>[4x]HHHHHHMSAIKPDMKINLRMEGNVNGHHFVIDGDGTGKPFEGKQSMDLEVKEGGPLPFAFDILTTAFHYGNRVFAEYPDHIQDYFKQSFPKGYSWERSLTFEDGGICIARNDI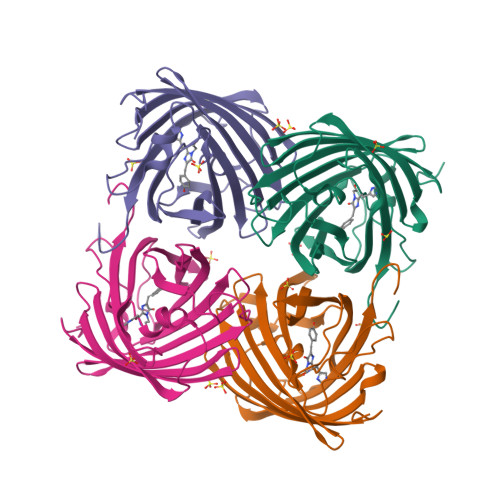TMEGDTFYNKVRFHGVNFPANGPVMQKKTLKWEPSTEKMYVRDGVLTGDITMALLLEGNAHYRCDSRTTYKAKEKGVKLPGYHLVDHCIEILSHDKDYNKVKLYEHAVAHSGLPDN N-[3-[(4R)-2-azanylidene-5,5-bis(fluoranyl)-4-methyl-1,3-oxazinan-4-yl]-4-fluoranyl-phenyl]-5-cyano-pyridine-2-carboxamide 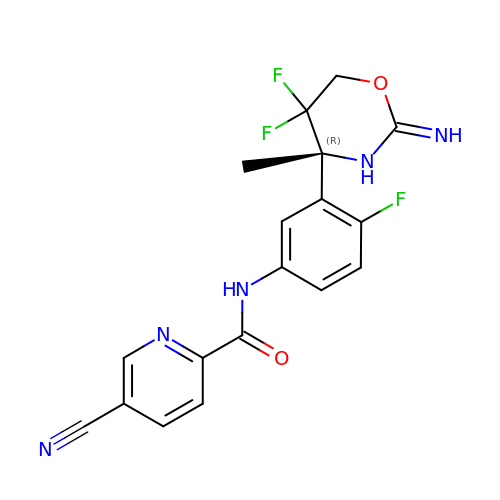| C18 H14 F3 N5 O2 | DVMUZHLUMHPCGZ-QGZVFWFLSA-N> AAPVAIQPTGYTLERVVILSRHGVRSPTKQTQLMNDVTPDTWPQWPVAAGELTPRGAQLVTLMGGFYGDYFRSQGLLAAGCPTDADIYAQADVDQRTRLTGQAFLDGIAPGCGLKVHYQADLKKVDPLFHPVDAGVCKLDSTQTHKAVEERLGGPLSELSKRYAKPFAQMGEILNFAASPYCKSLQQQGKTCDFANFAANKITVNKPGTKVSLSGPLALSSTLGEIFLLQNSQAMPDVAWHRLTGEDNWISLLSLHNAQFDLMAKTPYIARHKGTPLLQQIETALVLQRDAQGQTLPLSPQTKILFLGGHDTNIANIAGMLGLNWQLPQQPDNTPPGGGLVFELWQNPDNHQRYVAVKLFYQTMGQLRNAEKLDLKNNPAGRVPVAIDGCENSGDDKLCQLDTFQKKVAQAIEPACHI

The phytase APPA derived from Yersinia intermedia exhibits exceptional overall properties, including a high specific activity (3960 U/mg), excellent pH stability within the range of pH 2.5 to 10.0, and resistance to pepsin and trypsin digestion at 37 °C for 2 h, making it highly suitable for application in the feed industry. By hydrolyzing phytate—a compound that inhibits nutrient absorption found in animal feed—into inorganic phosphoric acid, it effectively reduces phosphorus excretion while enhancing mineral and protein digestion and absorption. However, the issue of heat resistance has emerged as a critical bottleneck hindering the industrial application of phytase due to the technical requirement of instantaneous high temperatures during feed pelletizing processes. The active site within the two domains typically consists of two conserved motifs: RHGXRXP in the N-terminal and HD in the C-terminal, with His and Asp serving as catalytic residues.

Among these variants, a clear increase in residual activity compared to that of APPA was observed for a variant with four mutations (APPA_Y51E/V86D/A323L/M359L, designated as APPAmut4). However, further verification through shaking flask fermentation revealed a progressive increase in expression levels of both APPA and APPAmut4 following induction, with the expression level of APPAmut4 surpassing that of APPA. The APPAmut4 exhibited optimal functionality at 55 °C, maintaining over half of its activity within the temperature range of 35 to 60 °C but becoming nearly inactive above 65 °C. Below 50 °C, the enzyme demonstrated stability; however, it experienced 45% decline in activity after a 2-min incubation and retained less than 10% activity following a 15-min incubation at 65 °C. Its half-life t1/2 value at 65 °C was approximately 3.4 min. Additionally, the T50 value was determined to be around 55.1 °C. The melting temperature, Tm, of the APPAmut4 (58.2 ± 0.9 °C), corresponding to the temperature at which a decrease in catalytic activity is observed, was found to be comparable to that of APPA (58.1 ± 0.9 °C). Therefore, we crystallized APPAmut4 (20 mg/ml) to determine its structural basis for the observed differences compared with the WT, resulting in crystals belonging to the orthorhombic space group P212121. B-factors analysis indicates that the α/β domain demonstrates relatively lower flexibility than the α-domain, particularly in the β-sheet region, suggesting a higher degree of rigidity. The N- and C-terminal regions, along with loop regions (residue 76–86, 119–128, 138–144, 235–246, 348–351, and 392–395), display flexibility which may negatively impact protein stability due to their limited interactions with other residues and disruption of noncovalent connections within complex networks.> MTNKQVEISMAEWDVMNIIWDKKSVSANEIVVEIQKYKEVSDKTIRTLITRLYKKEIIKRYKSENIYFYSSNIKEDDIKMKTAKTFLNKLYGGDMKSLVLNFAKNEELNNKEIEELRDILN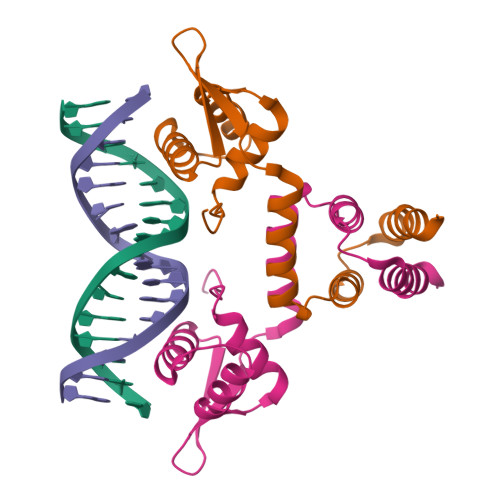DISKK dimethyl 3,3'-(6-methoxy-6-oxohex-1-ene-1,1-diyl)bis(5-cyano-6-methoxybenzoate) | C27 H26 N2 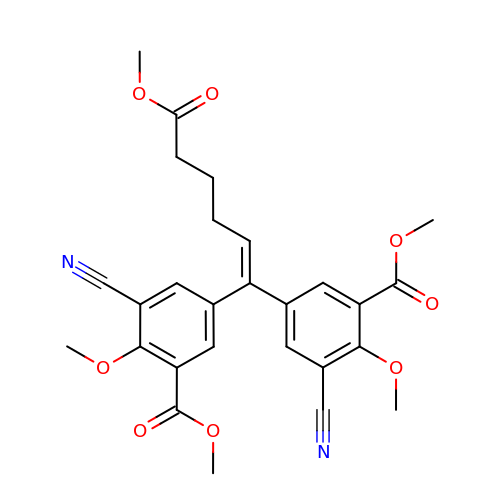O8 | KTXLKUASBPHAEE-UHFFFAOYSA-N2-(3-bromophenyl)quinoline-4-carboxylic acid | C16 H10 Br N O2 | 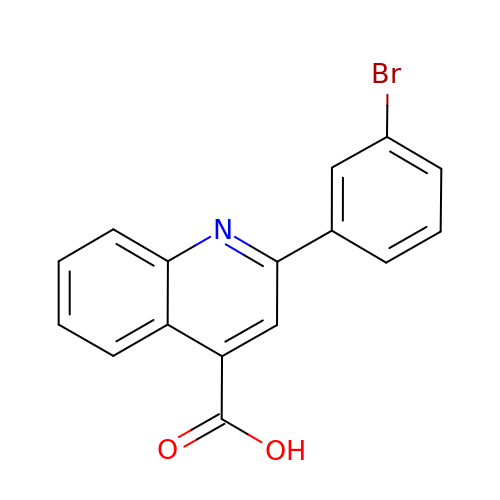KBIDGMKRLPPRNG-UHFFFAOYSA-N> XKGHPCDYPEWQ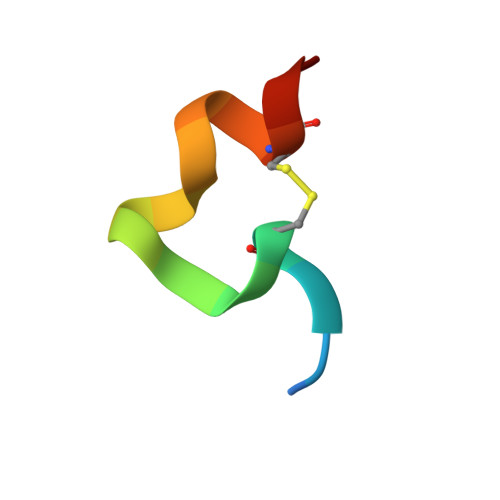WLCELX GUANIDINE | C H5 N3 | 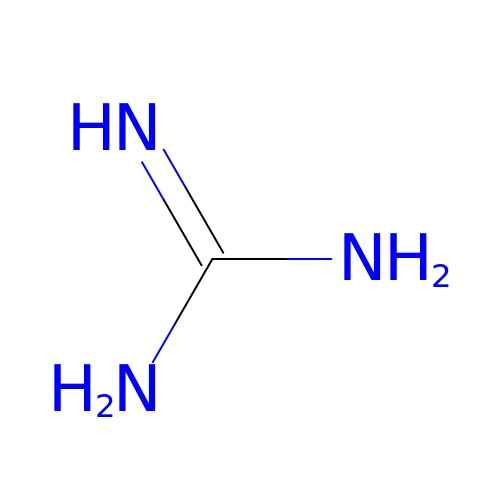ZRALSGWEFCBTJO-UHFFFAOYSA-N Pompe disease (also known as glycogen storage disease type 2 or acid maltase deficiency) is an autosomal recessive disorder caused by mutations in the gene that encodes the hydrolase acid α-glucosidase (GAA), member of glycoside hydrolase family GH311, and involved in the lysosomal breakdown of glycogen. GAA is synthesized as a 110 kDa glycoprotein, which is targeted to the lysosome via the mannose-6-phosphate receptor and undergoes in the late endosomal/lysosomal compartment a series of proteolytic and N-glycan processing events to yield a mature active form composed of four tightly associated peptides. A N-terminal trefoil Type-P domain is followed by a β-sheet domain, the catalytic (β/α)8 barrel bearing two inserts after β-strands β3 (insert I) and β4 (insert II), and proximal and distal β-sheet domains at the C-terminus. The narrow substrate-binding pocket of rhGAA is located near the C-terminal ends of β-strands of the catalytic (β/α)8 domain and shaped by a loop from the N-terminal β-sheet domain and both inserts I and II.

The proteolytic treatment yielded a polypeptide of ~5 kDa lower mass than the rhGAA precursor, which crystallized readily. This allowed us to collect the diffraction data extending to 1.9 Å and solve the structure of rhGAA by molecular replacement. In this study we employed in situ proteolysis to afford well-diffracting crystals of rhGAA and interestingly the crystallographic model we obtained corresponds to the mature forms of recombinant and placental GAA found in the endosome/lysosomal compartment. The overall architecture of rhGAA is similar to that of the human glycoside hydrolase family GH311 homologues, the intestinal brush-border enzymes maltase-glucoamylase (MGAM)22,23 and sucrase-isomaltase (SI)24. The precursor form of rhGAA contains ~14 kDa of carbohydrate and seven glycosylation sites have been predicted and characterized. We observed glycan structures of various lengths for five of them in the crystal structure, notably at N140, N233, N390, N470 and N652. We detected residual difference electron density at N882, insufficient to model a glycan structure, and did not observe difference electron density near N925. One of the peptide segments removed by proteolytic treatment (G116-M122) is specific to the lysosmal representatives of the GH31 enzyme family and its removal might be required for the generation of the secondary substrate-binding site in the trefoil Type-P domain.

> QCDVPPNSRFDCAPDKAITQEQCEARGCCYIPAKQGLQGAQMGQPWCFFPPSYPSYKLENLSSSEMGYTATLTRTTPTFFPKDILTLRLDVMMETENRLHFTIKDPANRRYEVPLETPRVHSRAPSPLYSVEFSEEPFGVIVHRQLDGRVLLNTTVAPLFFADQFLQLSTSLPSQYITGLAEHLSPLMLSTSWTRITLWNRDLAPTPGANLYGSHPFYLALEDGGSAHGVFLLNSNAMDVVLQPSPALSWRSTGGILDVYIFLGPEPKSVVQQYLDVVGYPFMPPYWGLGFHLCRWGYSSTAITRQVVENMTRAHFPLDVQWNDLDYMDSRRDFTFNKDGFRDFPAMVQELHQGGRRYMMIVDPAISSSGPAGSYRPYDEGLRRGVFITNETGQPLIGKVWPGSTAFPDFTNPTALAWWEDMVAEFHDQVPFDGMWIDMNEPSNFIRGSEDGCPNNELENPPYVPGVVGGTLQAATICASSHQFLSTHYNLHNLYGLTEAIASHRALVKARGTRPFVISRSTFAGHGRYAGHWTGDVWSSWEQLASSVPEILQFNLLGVPLVGADVCGFLGNTSEELCVRWTQLGAFYPFMRNHNSLLSLPQEPYSFSEPAQQAMRKALTLRYALLPHLYTLFHQAHVAGETVARPLFLEFPKDSSTWTVDHQLLWGEALLITPVLQAGKAEVTGYFPLGTWYDLQTVPIEALGSLPPPPAAPREPAIHSEGQWVTLPAPLDTINVHLRAGYIIPLQGPGLTTTESRQQPMALAVALTKGGEARGELFWDDGESLEVLERGAYTQVIFLARNNTIVNELVRVTSEGAGLQLQKVTVLGVATAPQQVLSNGVPVSNFTYSPDTKVLDICVSLLMGEQFLVSWC> MKRNPHFVSLTKNYLFADLQKRVAQFRLENPQHTVINLSIGDTTQPLNASVAEAFASSIARLSSPTTCRGYGPDFGLPALRQKLSEDFYRGFVDAKEIFISDGAKVDLFRLLSFFGPNQTVAIQDPSYPAYLDIARLTGAKEIIALPCLQENAFFPEFPEDTHIDILCLCSPNNPTGTVLNKDQLRAIVHYAIEHEILILFDAAYSTFISDPSLPKSIFEIPDARFCAIEINSFSKPLGFAGIRLGWTVIPQELTYADGHFVIQDWERFLSTTFNGASI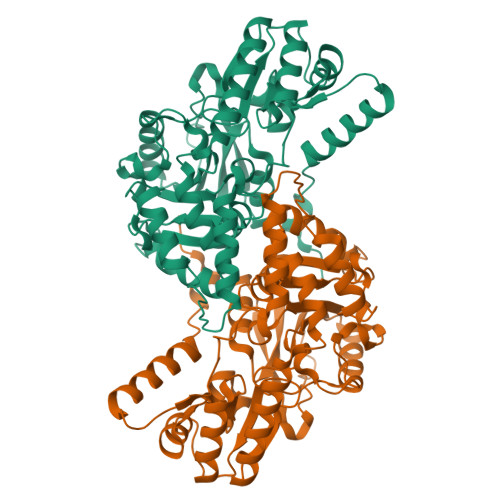PAQEAGVAGLSILPQLEAIHYYRENSDLLRKALLATGFEVFGGEHAPYLWVKPTQANISDRDLFDFFLREYHIAITPGIGFGRSGSGFVRFSSLGKREDILAACERLQMAPALQSHHHHHH>[2x]MELWLVRHGETLWNREGRLLGWTDLPLTAEGEAQARR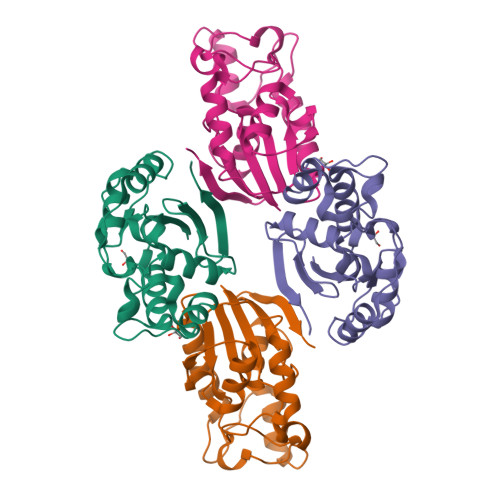LKGALPSLPAFSSDLLRARRTAELAGFSPRLYPELREIHFGALEGALWETLDPRYKEALLRFQGFHPPGGESLSAFQERVFRFLEGLKAPAVLFTHGGVVRAVLRALGEDGLVPPGSAVAVDWPRRVLVRLALDGEEATG The voltage-gated potassium channel AKT1 is responsible for primary K+ uptake in Arabidopsis roots. AKT1 is functionally activated through phosphorylation and negatively regulated by a potassium channel α-subunit AtKC1. AKT1 is the first characterized hyperpolarization-activated voltage-dependent K+ channel in Arabidopsis thaliana, which belongs to the Shaker K+ channel family. Each subunit can be divided into four parts: the transmembrane segments comprising S1–S6 and the pore loop; the C-linker which contains the helices A’B’C’D’; and the CNBD.

The electrophysiological results show that AtKC1 inhibits the channel activity of WT AKT1, the constitutively-active mutant Asp379Ala, and the phosphor-mimetics. Within expectation, the structure of AKT1-AtKC1 displays a 2-fold symmetric assembly at CPD. The overall structure of AKT1-AtKC1 is quite similar to WT AKT1, with root-mean-square deviations of 2.78 Å for 1753 aligned Cα atoms. The inner gate of the hetero-channel is also in closed state. Markedly, the C-linkers of AtKC1 resemble the “straight” C-linkers of AKT1 Mol I/I’, while the C-linkers of AKT1 exhibit the canonical “kinked” conformation as Mol II/II’. The “straight” C-linkers of AtKC1 may restrict the movement of adjacent C-linkers of AKT1. This structural observation mechanistically explains how AtKC1 exerted its inhibitory effect on AKT1. Different from WT AKT1, no extra densities that resemble loop1/1’ of AKT1 have been observed near the “straight” C-linker of AtKC1. This indicates the C-linkers of AtKC1 preferentially adopt a “straight” conformation, without the help of loop1/1’-like elements.

>[2x]MSTTTTEARSPLPLLLRRGRSSTALSASTAEARSPLSILQFRRRSSKDVRNITSVSSSLLPAFGTFIEDDNPSSKPFIVLHFDRRYRLWELFLVILVGYSAWASLFELAFEKAAEGALLTIDLVVDFFFAVDIILTFFVSYLDNTTYLNVTDHKLIAKRYLKSVAFVMDVASTLPIQFIYKTITGDVGRGQAFGFLNLLRLWRLRRVAELFKRLEKDAHFNYFVIRVIKLLCVTIFWIHLAGCILYWIAYHYPRPTDTWIGSQVEDFKERSVWLGYTYSMYWSIVTLTTVGYGDLHAVNSREKTFNMFYMLFNIGLTSYIIGIMTNLVVHGALRTFAMRSAINDILRYTSKNRLPDTMREQMLAHMQLKFKTAELRQEEVLQDLPKAIRSSINQHLFRSIIEEAYLFKGFPEGLLVQLVSQIQAEYFPPKMEIILQNEIPTDFYVIVSGGVDIIASKGVSEQVLAKLGPGSMAGEIGVVFNIPQPFTVRTRRLSQVIRIGHHKFKEMVQSDNDVDAKMIIANFMTYLKGLNDELKKEIPFLRDLLDDADAQVQETVQSEETPQSNDEEIVTVSRHENGQIEERRREGVPKRVIIHGQAPPNQDNKNNGDSNGRLIILPDSIQLLFDLAEKKLGKRGSTIAMADGAHVEQIDALRENDHLYIF;>MRGGALLCGQVQDEIEQLSRESSHFSLSTGILPSLGARSNRRVKLRRFVVSPYDHKYRIWEAFLVVLVVYTAWVSPFEFGFLRKPRPPLSITDNIVNAFFAIDIIMTFFVGYLDKSTYLIVDDRKQIAFKYLRSWFLLDLVSTIPSEAAMRISSQSYGLFNMLRLWRLRRVGALFARLEKDRNFNYFWVRCAKLVCVTLFAVHCAACFYYLIAARNSNPAKTWIGANVANFLEESLWMRYVTSMYWSITTLTTVGYGDLHPVNTKEMIFDIFYMLFNLGLTAYLIGNMTNLVVHGTSRTRNFRDTIQAASNFAHRNHLPPRLQDQMLAHLCLKYRTDSEGLQQQETLDALPKAIRSSISHFLFYSLMDKVYLFRGVSNDLLFQLVSEMKAEYFPPKEDVILQNEAPTDFYILVNGTADLVDVDTGTESIVREVKAGDIIGEIGVLCYRPQLFTVRTKRLCQLLRMNRTTFLNIIQANVGDGTIIMNNLLQHLKEMNDPVMTNVLLEIENMLARGKMDLPLNLCFAAIREDDLLLHQLLKRGLDPNESDNNGRTPLHIAASKGTLNCVLLLLEYHADPNCRDAEGSVPLWEAMVEGHEKVVKVLLEHGSTIDAGDVGHFACTAAEQGNLKLLKEIVLHGGDVTRPRATGTSALHTAVCEENIEMVKYLLEQGADVNKQDMHGWTPRDLAEQQGHEDIKALFREKLHERRVHIETSSSVPILKTGIRFLGRFTSEPNIRPASREVSFRIRETRARRKTNNFDNSLFGILANQSVPKNGLATVDEGRTGNPVRVTISCAEKDDIAGKLVLLPGSFKELLELGSNKFGIVATKVMNKDNNAEIDDVDVIRDGDHLIFATDS[2x]> AMDKSAKAPVITI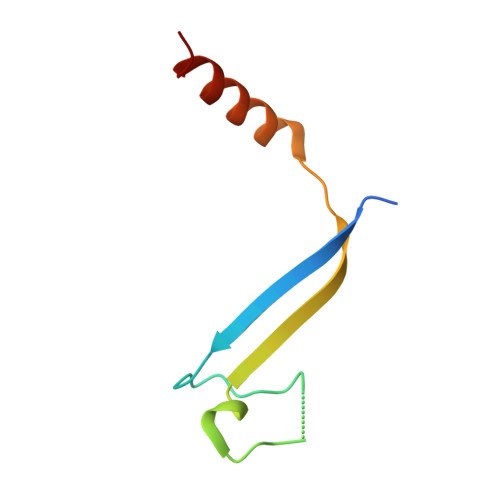FDHRGCSRAPKEYTGSKASGQDDEMMVKAQSVKIAVSDGVAESVLKDSLSVMHK> MAAFKPNSINYILGLDIGIASVGWAMVEIDEEENPIRLIDLGVRVFERAEVPKTGDSLAMARRLARSVRRLTRRRAHRLLRTRRLLKREGVLQAANFDENGLIKSLPNTPWQLRAAALDRKLTPLEWSAVLLHLIKHRGYLSQRKNEGETADKELGALLKGVAGNAHALQTGDFRTPAELALNKFEKESGHIRNQRSDYSHTFSRKDLQAELILLFEKQKEFGNPHVSGGLKEGIETLLMTQRPALSGDAVQKMLGHCTFEPAEPKAAKNTYTAERFIWLTKLNNLRILEQGSERPLTDTERATLMDEPYRKSKLTYAQARKLLGLEDTAFFKGLRYGKDNAEASTLMEMKAYHAISRALEKEGLKDKKSPLNLSPELQDEIGTAFSLFKTDEDITGRLKDRIQPEILEALLKHISFDKFVQISLKALRRIVPLMEQGKRYDEACAEIYGDHYGKKNTEEKIYLPPIPADEIRNPVVLRALSQARKVINGVVRRYGSPARIHIETAREVGKSFKDRKEIEKRQEENRKDREKAAAKFREYFPNFVGEPKSKDILKLRLYEQQHGKCLYSGKEINLGRLNEKGYVEIDHALPFSRTWDDSFNNKVLVLGSENQNKGNQTPYEYFNGKDNSREWQEFKARVETSRFPRSKKQRILLQKFDEDGFKERNLNDTRYVNRFLCQFVADRMRLTGKGKKRVFASNGQITNLLRGFWGLRKVRAENDRHHALDAVVVACSTVAMQQKITRFVRYKEMNAFDGKTIDKETGEVLHQKTHFPQPWEFFAQEVMIRVFGKPDGKPEFEEADTLEKLRTLLAEKLSSRPEAVHEYVTPLFVSRAPNRKMSGQGHMETVKSAKRLDEGVSVLRVPLTQLKLKDLEKMVNREREPKLYEALKARLEAHKDDPAKAFAEPFYKYDKAGNRTQQVKAVRVEQVQKTGVWVRNHNGIADNATMVRVDVFEKGDKYYLVPIYSWQVAKGILPDRAVVQGKDEEDWQLIDDSFNFKFSLHPNDLVEVITKKARMFGYFASCHRGTGNINIRIHDLDHKIGKNGILEGIGVKTALSFQKYQIDELGKEIRPCRLKKRPPVR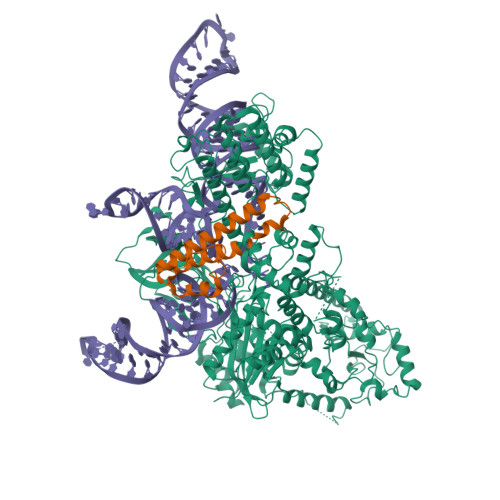;> MKITSSNFATIATSENFAKLSVLPKNHREPIKGLFKSAVEQFSSARDFFKNENYSKELAEKFNKEAVNEAVEKLQKAIDLAEKQGIQF> MPNLFPQSETFETVELKNNDENELD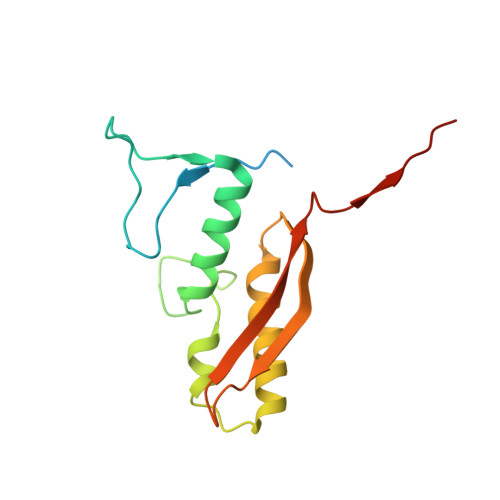LKGSFLFDFEKGEFVKNADGTLKKCDKVQAYKQWCQKAILTPRYKKAAYTNIYGSEIKDLIASNLSQSAKELEITRLIKETILVHPYTKEVGEFSFNWLENSRLVEYEFDVLTIDDENIVIDGNIKR4-[3-(4-fluorophenyl)-1-methyl-1H-pyrazol-4-yl]-6-methyl-6,7-dihydro-5H-pyrrolo[3,4-b]pyridin-5-one | C18 H15 F N4 O | 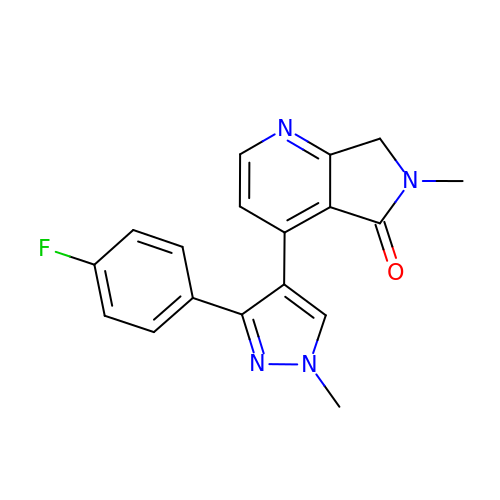NGDXEOHYWJHBTJ-UHFFFAOYSA-N> AVVEFAGSAFEVDEDGFLNA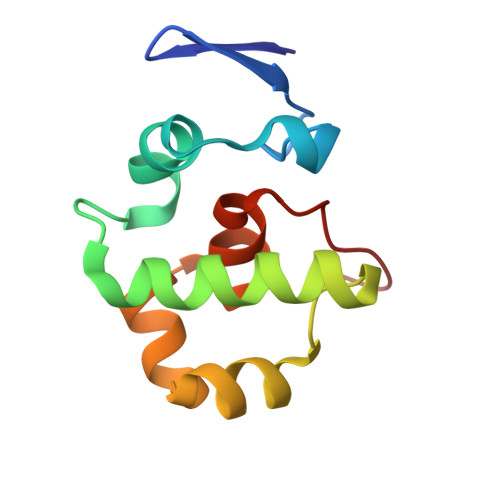FDDWCPEWVKYAKGSEGIGAGSADHQKIIDFLQDYYKANGIAPMVRILSKVTGFKLKQIYELFPSGPGKGACKMAGLPKPTGCV>GIGDPVTCLKSGAICHPVFCPRRYKQIGTCGL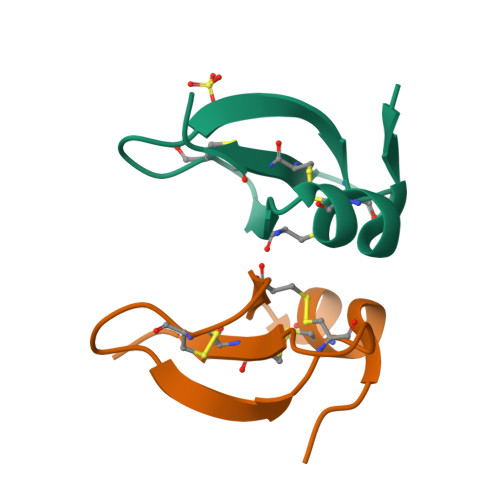PGTKCCKKP[16x]> GMNLTELMERIPHLREILNIVREAFKDYDDPAHDISHTFRVME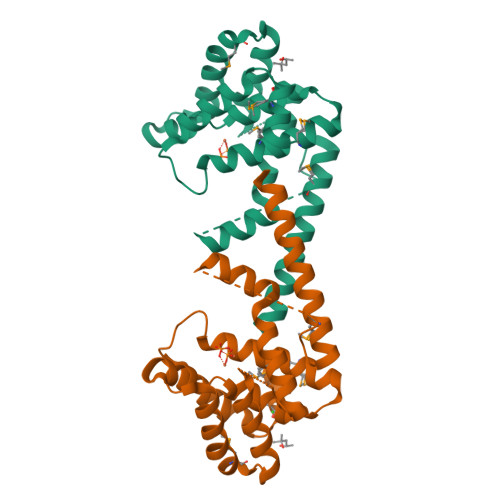NASEIASREKCDLQKAIIAALLHDIKRPHEALTGVDHAESGAEYASGLLPTMGFDISFVAEVSKAIRSHRYSGGLTPTSLTGKILQDADRLDAIGAVAIARVFSYSGKTGTPLHSLQFSPRSSYSGNSRSSINHFHEKILKIRPETFWTETARKMAEDRYSFVVEFVQRFLAEWGQI With the exception of a subset of lipoproteins that carry a transport avoidance signature and remain in the inner membrane, the majority of lipoproteins are destined for the outer membrane. Their transport is directed by the Lol system that comprises the inner membrane transporter LolCDE, the periplasmic chaperone LolA, and the outer membrane receptor LolB, itself a lipoprotein. Following maturation on the inner membrane and extraction by the LolCDE transporter, lipoproteins are passed to the chaperone LolA that carries them across the periplasm prior to insertion into the outer membrane by the LolB receptor. LolA and LolB share structural homology, both being incomplete β-barrels with a central hydrophobic cavity closed by an alpha helical lid, but perform distinct functions. Here, we present the crystal structure of LolA in complex with a lipoprotein, providing a molecular description of the interaction and a rationale for the capacity of the chaperone protein to transport evolutionarily divergent lipoproteins.

Thus, to capture a LolA–lipoprotein intermediate favorable for structural studies, we introduced a tobacco etch virus (TEV) protease cleavage site in the N-terminal region of Pal to permit targeted removal of the lipoprotein linker and globular domain. We determined the crystal structure of LolA–Pal13 at 1.83-Å resolution. The protein complex crystallized in space group I4 with one molecule per asymmetric unit. We resolved density for the triacylated cysteine but not for the rest of the peptide chain, suggesting that LolA does not make specific interactions with the lipoprotein amino acid chain, consistent with our demonstration that transfer to LolB can occur in the absence of the lipoprotein globular domain. The three acyl chains of the ligand are inserted deeply in the U-shaped cavity of LolA with electron density compatible with 16-carbon chains, consistent with the predominant species in E. coli lipoproteins. The acyl chains pack together with R1 and R2 running straight down and R3 packed against the other two chains at ∼45° angle. The lipoprotein triacyl group is stabilized by van der Waals (VDW) interactions with multiple residues forming the hydrophobic cavity of LolA. Interestingly, two polar interactions between the carbonyl group of the R2 ester linkage and the side chains of both S150 and Y152 also stabilize the lipoprotein. Here, we show that the triacyl moiety opens the deepest part of the LolA pocket by a further 1.5-fold, increasing the cavity volume to ∼1,400 Å3. Relative to apo LolA, the helix is displaced by about 9 Å, a motion required for the accommodation of the three acyl chains deep inside the cavity.

> DAASDLKSRLDKVSSFHASFTQKVTDGSGAAVQEGQGDLWVKRPNLFNWHMTQPDESILVSDGKTLWFYNPFVEQATATWLKDATGNTPFMLIARNQSSDWQQYNIKQNGDDFVLTPKASNGNLKQFTINVGRDGTIHQFSAVEQDDQRSSYQLKSQQNGAVDAAKFTFTPPQGVTVDDQRKGSWSHPQFEK N-[(5S,9S,10S,13S)-9-hydroxy-5,10-bis(2-methylpropyl)-4,7,12,16-tetraoxo-3,6,11,17-tetraazabicyclo[17.3.1]tricosa-1(23),19,21-trien-13-yl]-3-(naphthalen-1-yl)-2-(naphthalen-1-ylmethyl)propanamide 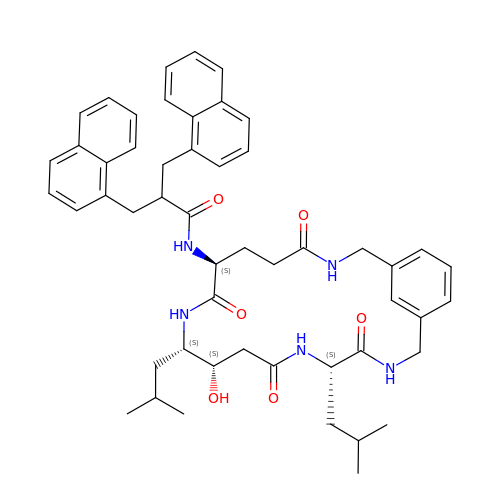| C51 H61 N5 O6 | KFCMUWOMPCWWCH-AXYJRABVSA-N> RHSRRAIAAETVEILERGRYTAPSGRVVPIADHVAQAVRGTRLYRPEKLAVLLEGLGAASDGAPTRIEVTEETTLAAARRLTGAAGDQVACLNFASAEHPGGGFLSGAHAQEAGLARSSGLYASLRAVPQFYAFHHRQRDPLYSDHLIYSPGVPVFRDDAGRLLEEPYRVAFLTSPAPNRRAIGDLRTVEEIGRVLRGRAAKVLAAARHHGHRRLVLGAWGCGVFGNDPAQVAE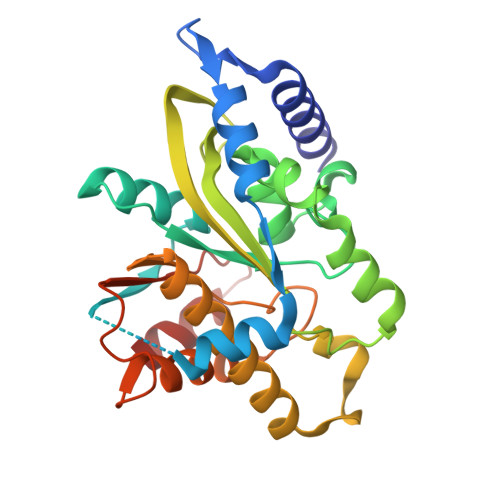TFAGLLLDGGPFAGRFAHVVFAVWDTAPGAPRHAAFARRFGSL> MAKKTSSGRGKLPPGPTPLPVIGNILQIGIKDISKSLTNLSKVYGPVFTLYFGLKPIVVLHGYEAVKEALIDLGEEFSGRGIFPLAERANRGFGIVFSNGKKWKEIRRFSLMTLRNFGMGKRSIEDRVQEEARCLVEELRKTKASPCDPTFILGCAPCNVICSIIFHKRFDYKDQQFLNLMEKLNENIKILSSPWIQICNNFSPIIDYFPGTHNKLLKNVAFMKSYILEKVKEHQESMDMNNPQDFIDCFLMKMEKEKHNQPSEFTIESLENTAVDLFGAGTETTSTTLRYALLLLLKHPEVTAKVQEEIERVIGRNRSPCMQDRSHMP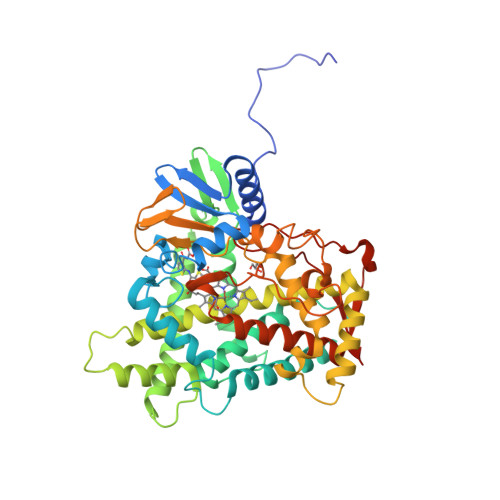YTDAVVHEVQRYIDLLPTSLPHAVTCDIKFRNYLIPKGTTILISLTSVLHDNKEFPNPEMFDPHHFLDEGGNFKKSKYFMPFSAGKRICVGEALAGMELFLFLTSILQNFNLKSLVDPKNLDTTPVVNGFASVPPFYQLCFIPIHHHH>MKTLSQAQSKTSSQQFSFTGNSSANVIIGNQKLTINDVARVARNGTLVSLTNNTDILQGIQASCDYINNAVESGEPIYGVTSGFGGMANVAISREQASELQTNLVWFLKTGAGNKLPLADVRAAMLLRANSHMRGASGIRLELIKRMEIFLNAGVTPYVYEFGSIGASGDLVPLSYITGSLIGLDPSFKVDFNGKEMDAPTALRQLNLSPLTLLPKEGLAMMNGTSVMTGIAANCVYDTQILTAIAMGVHALDIQALNGTNQSFHPFIHNSKPHPGQLWAADQMISLLANSQLVRDELDGKHDYRDHELIQDRYSLRCLPQYLGPIVDGISQIAKQIEIEINSVTDNPLIDVDNQASYHGGNFLGQYVGMGMDHLRYYIGLLAKHLDVQIALLASPEFSNGLPPSLLGNRERKVNMGLKGLQICGNSIMPLLTFYGNSIADRFPTHAEQFNQNINSQGYTSATLARRSVDIFQNYVAIALMFGVQAVDLRTYKKTGHYDARACLSPATERLYSAVRHVVGQKPTSDRPYIWNDNEQGLDEHIA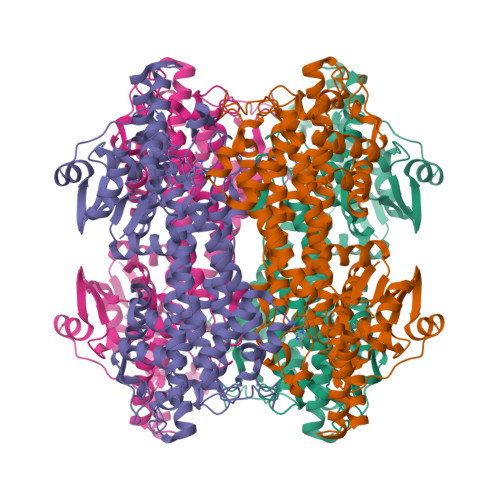RISADIAAGGVIVQAVQDILPCLH[4x]> GSPPKGPELSLASIHVPLESIKPSSALPVTAYDKNGFRILFHFAKECPPGRPDVLVVVVSMLNMAPLPVKSIVLQAAAPKSMKVKLQPPSGTELSPFSPI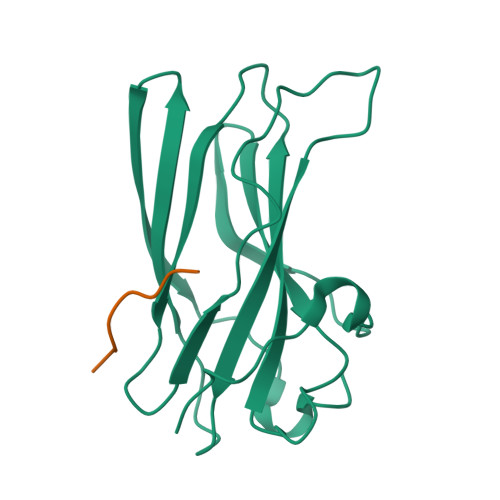QPPAAITQVMLLANPLKEKVRLRYKLTFALGEQLSTEVGEVDQFPPVEQWGNL;> DESDFGPLVGADS> MHHCKRYRSPEPDPYLSYRWKRRRSYSREHEGRLRYPSRREPPPRRSRSRSHDRLPYQRRYRERRDSDTYRCEERSPSFGEDYYGPSRSRHRRRSRERGPYRTRKHAHHCHKRRTRSCSSASSRSQQSSKRSSRSVEDDKEGHLVCRIGDWLQEDYEIVGNLGEGTFGKVVECLDHARGKSQVALKIIRNVGKYREAAR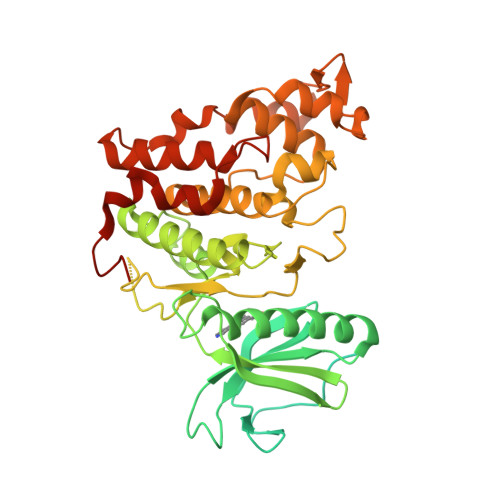LEINVLKKIKEKDKENKFLCVLMSDWFNFHGHMCIAFELLGKNTFEFLKENNFQPYPLPHVRHMAYQLCHALRFLHENQLTHTDLKPENILFVNSEFETLYNEHKSCEEKSVKNTSIRVADFGSATFDHEHHTTIVATRHYRPPEVILELGWAQPCDVWSIGCILFEYYRGFTLFQTHENREHLVMMEKILGPIPSHMIHRTRKQKYFYKGGLVWDENSSDGRYVKENCKPLKSYMLQDSLEHVQLFDLMRRMLEFDPAQRITLAEALLHPFFAGLTPEERSFHTSRNPSR> DEELEEIKKETGFSHSQITRLYSRFTSLDKGENGTLSREDFQRIPELAINPLGDRIINAFFPEGEDQVNFRGFMRTLAHFRPIEDNEKSKDVNGPEPLNSRSNKLHF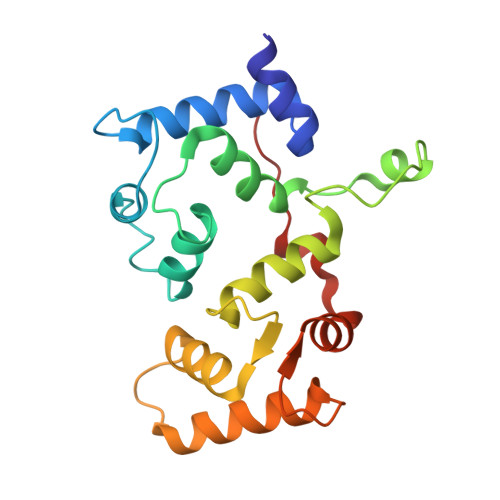AFRLYDLDKDEKISRDELLQVLRMMVGVNISDEQLGSIADRTIQEADQDGDSIASFTEFVKVLEKVDVEQKMSIRFLH> ADNEVTAEGGKLVQELVYDHSAIPVAPVVETQAEQPEVPVSLVATRKNDTGHLATKWYDFAKISLSNPANMNWTTLTIDPYNNVTLSRDGESMVLPWRRNVWTTGSKSIGYIRTMVAQINIPRPPQISGVLEVKDSINNSSISLVEFGGKVEIPIIPKVMNGLATTASLPRHRLNPWMRTAESKVELQYRIIAFNRTSDIADL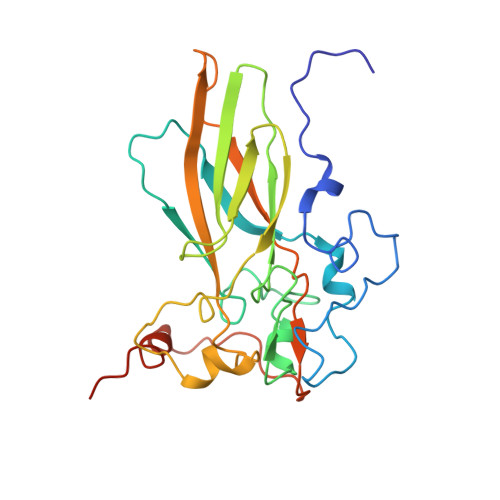NVSVLLRPGDSQFQLPMKPDNNVDTRHFELVEALMYHYDSLRIRGEEQ> NF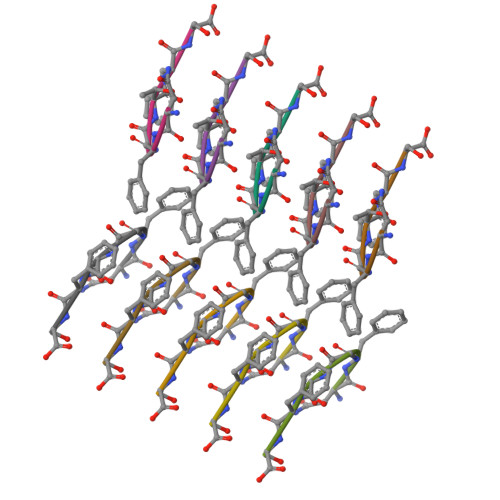GTFS> MAHEILIAETEAFLKNVAPETRTAIISAITGGKSACKSAAKLIKNEHLPLMSGEATTMHIVMRCLYPEIKPW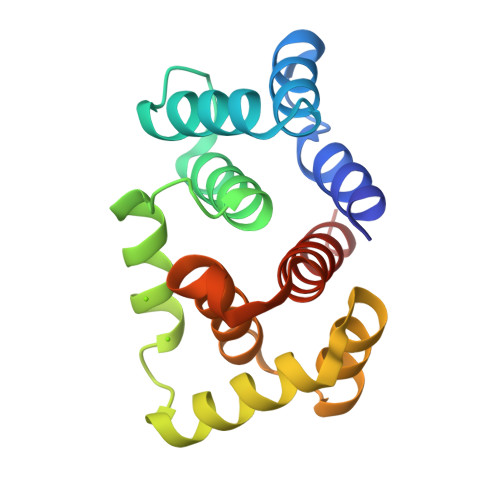KKASDMLNKATSSLKKSEGRDIRKQMKAAGDFLGVESMMKMRAFRDDQIMEMVEEVYDHPDDYTPDIRIGTITAWLRCKNKKS>MTQRLKDKLAVITGGANGIGRAIAERFAVEGADIAIADLVPAPEAEAAIRNLGRRVLTVKCDVSQPGDVEAFGKQVISTFGRCDILVNNAGIYPLIPFDELTFEQWKKTFEINVDSGFLMAKAFVPGMKRNGWGRIINLTSTTYWLKIEAYTHYISTKAANIGFTRALASDLGKDGITVNAIAPSLVRTATTEASALSAMFDVLPNMLQAIPRLQVPLDLTGAAAFLASD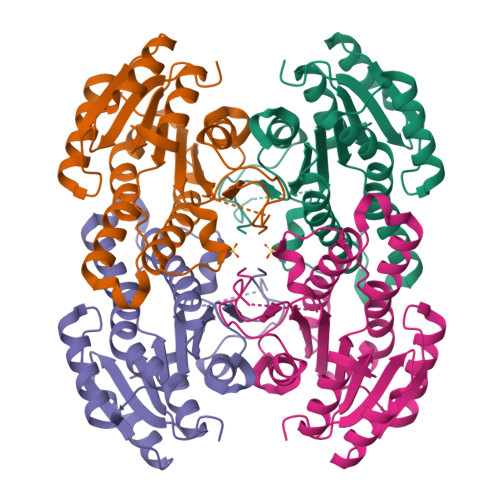DASFITGQTLAVDGGMVRH[4x]>SMSLELQEHCSLKPYNTFGIDVRARLLAHARDEADVREALALARERGLPLLVIGGGSNLLLTRDVEALVLRMASQGRRIVSDAADSVLVEAEAGEAWDPFVQWSLERGLAGLENLS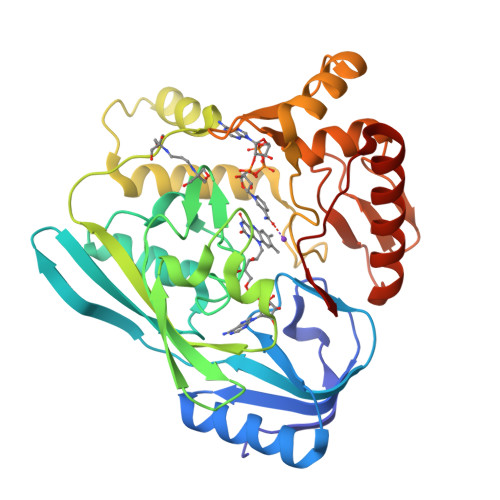LIPGTVGAAPMQNIGAYGVELKDVFDSLTALDRQDGTLREFDRQACRFGYRDSLFKQEPDRWLILRVRLRLTRRERLHLDYGPVRQRLEEEGIASPTARDVSRVICAIRREKLPDPAVLGNAGSFFKNPLVDATQAERLRQAFPDLVGYPQADGRLKLAAGWLIDKGGWKGFRDGPVGVHAQQALVLVNHGGATGAQVRALAERIQEDVRRRFGVELEPEPNLY[4x]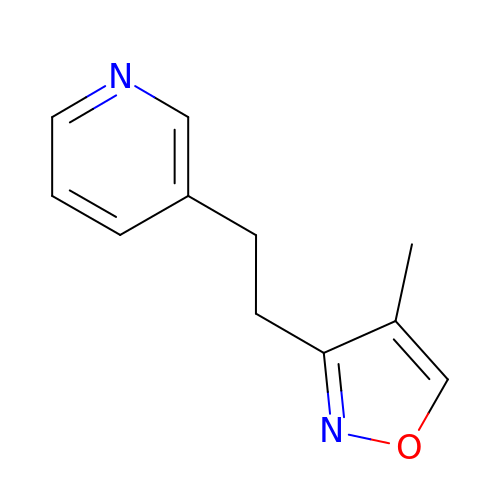3-[2-(4-methyl-1,2-oxazol-3-yl)ethyl]pyridine | C11 H12 N2 O | ZUKCCHMCKBWNOY-UHFFFAOYSA-N>[2x]MEPLKVEKFATANRGNGLRAVTPLRPGELLFRSDPLAYTVCKGSRGVVCDRC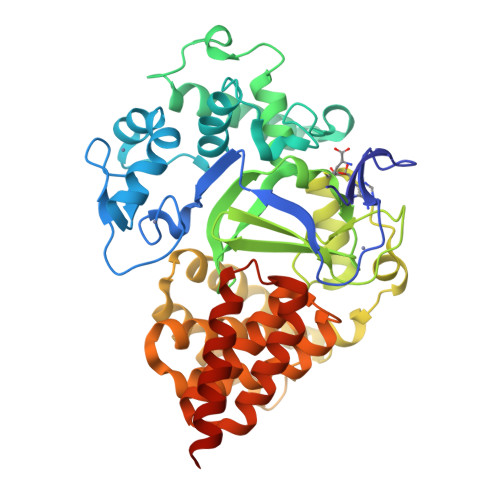LLGKEKLMRCSQCRVAKYCSAKCQKKAWPDHKRECKCLKSCKPRYPPDSVRLLGRVVFKLMDGAPSESEKLYSFYDLESNINKLTEDRKEGLRQLVMTFQHFMREEIQDASQLPPAFDLFEAFAKVICNSFTICNAEMQEVGVGLYPSISLLNHSCDPNCSIVFNGPHLLLRAVRDIEVGEELTICYLDMLMTSEERRKQLRDQYCFECDCFRCQTQDKDADMLTGDEQVWKEVQESLKKIEELKAHWKWEQVLAMCQAIISSNSERLPDINIYQLKVLDCAMDACINLGLLEEALFYGTRTMEPYRIFFPGSHPVRGVQVMKVGKLQLHQGMFPQAMKNLRLAFDIMRVTHGREHSLIEDLILLLEECDANIRASLEHHHHHH> 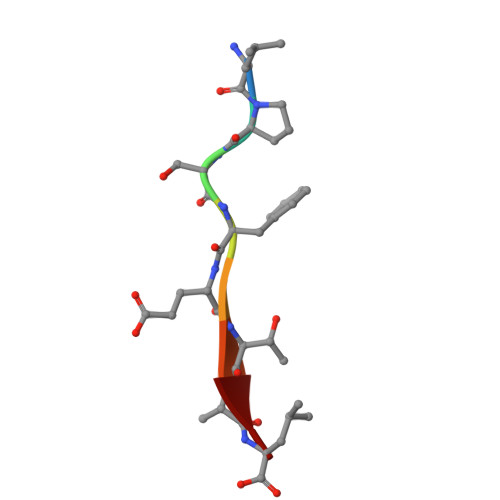LPSFETAL>MADNMTTTQIEVGPGATNATINFEAGILECYERFSWQRALDYPGQDRLHRLKRKLESRIKTHNKSEPENKRM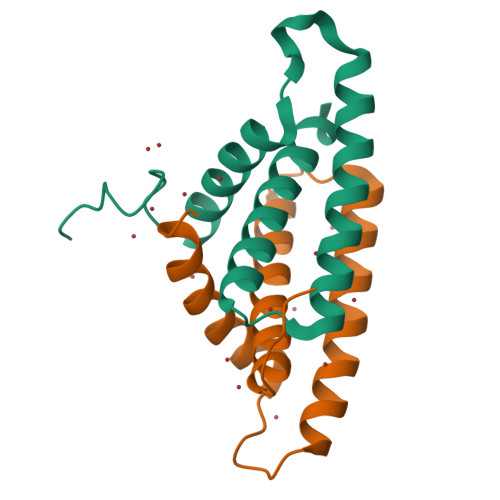SLEERKAIGVKMMKVLLFMDPSAGIEGFEPY[2x]>NPTSLTDVRVDKAVNFIKPEVSGVAEIQTVTGLSPSTSYLLTPAFLEQNFQSEAGIYILSATPVEG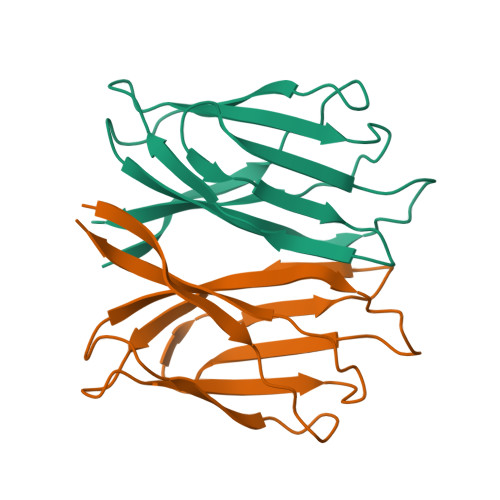EGTISINMDPTVTTVSGFIKVKTDTFGTFDLSVVLTTASKKQTTGFNIIAATS[2x]> GSGSGSMQSTSNHLWLLSDILGQGATANVFRGRHKKTGDLFAIKVFNNISFLRPVDVQMREFEVLKKLNHKNIVKLFAIEEETTTRHKVLIMEFCPCGSLYTVLEEPSNAYGLPESEFLIVLRDVVGGMNHLRENGIVHRNIKPGNIMRVIGEDGQSVYKLTDFGAARELEDDEQFVSLYGTEEYLHPDMYERAVLRKDHQKKYGATVDLWSIGVTFYHAATGSLPFRPFEGPRRNKEVMYKIITGKPSGAISGVQKAENGPIDWSGDMPVSCSLSRGLQVLLTPVLANILEADQEKCWGFDQFFAETSDILHRMVIHVFSLQQMTAHKIYIHSYNTATIFHELVYKQTKIISSNQELIYEGRRLVLEPGRLAQHFPKTTEENPIFVVSREPLNTIGLIYEKISLPKVHPRYDLDGDASMAKAITGVVCYACRIASTLLLYQELMRKGIRWLIELIKDDYNETVHKKTEVVITLDFCIRNIEKTVKVYEKLMKINLEAAELGEISDIHTKLLRLSSSQGTIETSLQDIDSRLSPGGSLADAWAHQEGTHPKDRNVEKLQVLLNCMTEIYYQFKKDKAERRLAYNEEQIHKFDKQKLYYHATKAMTHFTDECVKKYE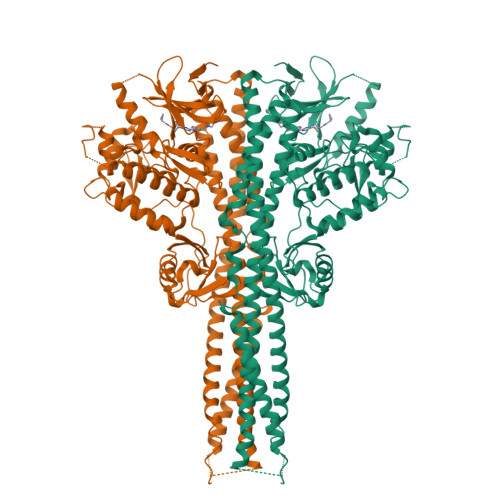AFLNKSEEWIRKMLHLRKQLLSLTNQCFDIEEEVSKYQEYTNELQET>[8x]GHMSTLLINQPQYAWLKELGLREENEGVYNGSWGGRGEVITTYCPANNEPIARVRQASVADYEETVKKAREAWKIWADIPAPKRGEIVRQIGDALREKIQVLGSLVSLEMGKILVEGVGEVQEYVDICDYAVGLSRMIGGPILPSERSGHALIEQWNPVGLVGIITAFNFPVVVYGWNNAIAMICGNVCLWKGAPTTSLISVAVTKIIAKVLEDNKLPGAICSLTCGGADIGTAMAKDERVNLLSFTGSTQVGKQVGLMVQERFGRSLLEL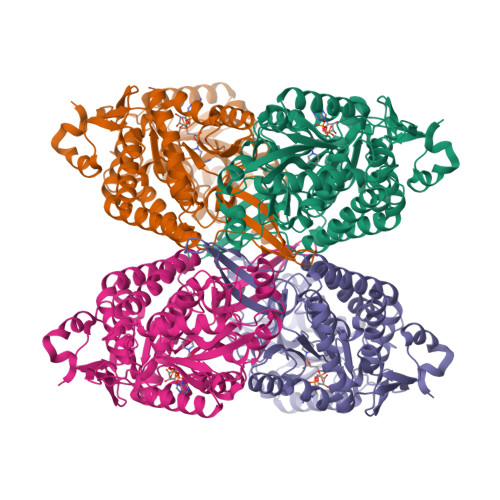GGNNAIIAFEDADLSLVVPSALFAAVGTAGQRCTTARRLFIHESIHDEVVNRLKKAYAQIRVGNPWDPNVLYGPLHTKQAVSMFLGAVEEAKKEGGTVVYGGKVMDRPGNYVEPTIVTGLGHDASIAHTETFAPILYVFKFKNEEEVFAWNNEVKQGLSSSIFTKDLGRIFRWLGPKGSDCGIVNVNIPTSGAEIGGAFGGEKHTGGGRESGSDAWKQYMRRSTCTINYSKDLPLAQGIKFQ>GSHMSVSGSERSAEGNRKKRVVIVGGGTAGWMTASYLTAAFGDRVDLTVVESAQIGTIGVGEATFSDIRHFFEFLRLEES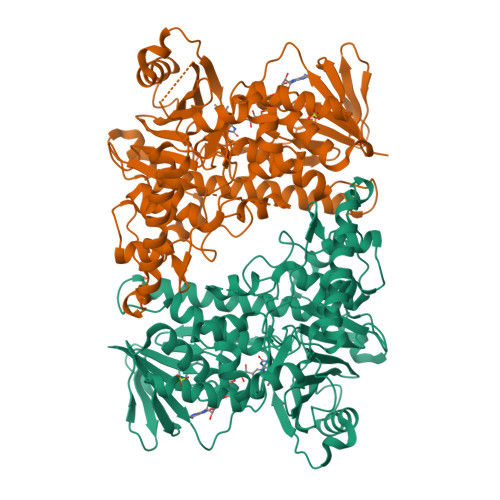DWMPECNATYKLAVRFENWREPGHHFYHPFEQMSSVDGFPLSDWWLRNPTTSRFDKDSFVMTSLCDAGVSPRYLDGSLIDQDFVEQERDDDSARSTIAEYQGAQFPYAYHFEAHLLAKYLTGYATRRGTRHIVDNVVDVALDERGWISHVRTEEHGDLEADLFVDCTGFRGLLLNKALGEPFVSYQDTLPNDSAVALQVPLDMEREPIRPCTTATAQEAGWIWTIPLISRVGTGYVYASDYTTPEQAERVLRDFVGPAAADVPANHIKMRIGRSRRSWVNNCVGVGLSSGFVEPLESTGIFFIHHAIEQIVKYFPSGGAGDDRLRELYNRSVGHVMDGVREFLVLHYRSAKRADNQYWKDTKTRTVPDSLAERIEFWKHKVPDAETVYPYYHGLPPYSYNCILLGMGGIDVNYSPALDWANEKAALAEFERIRVKAEKLVQELPTQNEYFAAMRAGR[2x]>SFLHVGKMGFVVTMLKLIQKKLLDKTCDQVMEFSWSALWNITDETPDNCEMFLNFNGMKLFLDCLKEFPEKQELHRNMLGLLGNVAEVKELRPQLMTSQFISVFSNLLESKADGIEVSYNACGVLSHIMFDGPEAWGVCEPQREEVEERMWAAIQSWDINSRRNINYRSFEPILRLLPQGISPVSQHWATWALYNLVSVYPDKYCPLLIKEGGMPLLRDIIKMATARQETKEMARKVIEHCSNFKEENMD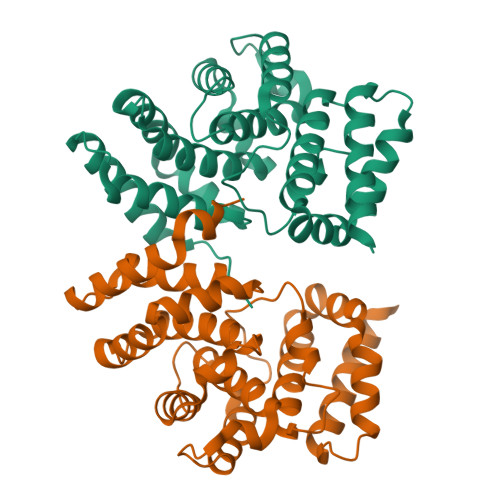TSR[4x]>[2x]GSTQEEIENLPAFPREKLTLRLLLGSGAFGEVYEGTAVDILGVGSGEIKVAVKTLKKGSTDQEKIEFLKEAHLMSKFNHPNILKQLGVCLLNEPQYIILELMEGGDLLTYLRKARMATFYGPLLTLVDLVDLCVDISKGCVYLERMHFIHRDLAARNCLVSVKDYTSPRIVKIGDFGLARDIYKNDYYRKRGEGLLPVRWMAPESLMDGIFTT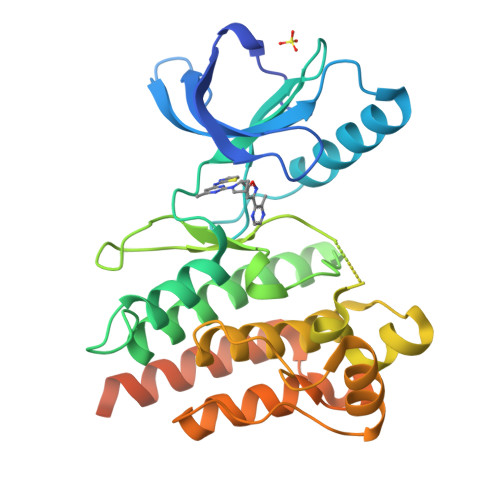QSDVWSFGILIWEILTLGHQPYPAHSNLDVLNYVQTGGRLEPPRNCPDDLWNLMTQCWAQEPDQRPTFHRIQDQLQLFRNFFLNSIYKSRDEANNSGVINESFEGEDGDVICLNSDLE> TRFTEEYQLFEELGKGAFSVVRRCVKVLAGQEYAAKIINTKKLSARDHQKLEREARICRLLKHPNIVRLHDSISEEGHHY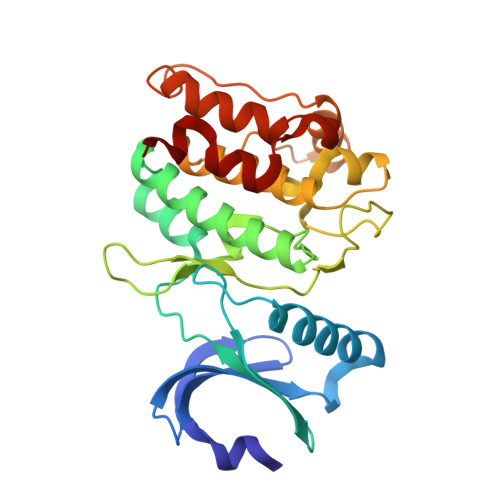LIFDLVTGGELFEDIVAREYYSEADASHCIQQILEAVLHCHQMGVVHRNLKPENLLLASKLKGAAVKLADFGLAIEVEGEQQAWFGFAGTPGYLSPEVLRKDPYGKPVDLWACGVILYILLVGYPPFWDEDQHRLYKQIKAGAYDFPSPEWDTVTPEAKDLINKMLTINPSKRITAAEALKHPWISHR>MSIKTNVEEILEDIKKYSPYPEKVKLVAVTKYSSVEDIEKFLETGQNICGENKVQVIKDKIEYFKEKNKKIKWHFIGNLQKNKVKYIIDDVDLIHSVNKLSLAQEINKKAEQSSKIMDVLLEINVYGEESKQGYSLDELKCDIIELQNLKNLNIIGVMTMAPFTDDEKILR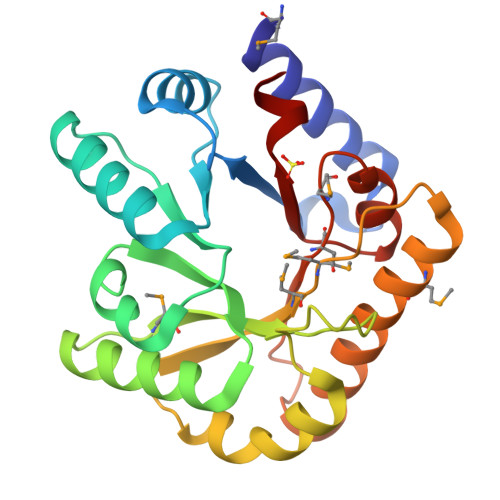MVFSELRKIKDELNKEYFNNNLTELSMGMSNDYKIALQEGSTFIRVGTKIFK[3x]> MRGSFVEMVDNLRGKSGQGYYVEMTVGSPPQTLNILVDTGSSNFAVGAAPHPFLHRYYQRQLSSTYRDLRKGVYVPYTQGKWEGELGTDLVSIPHGPNVTVRANIAAITESDKFFINGSNWEGI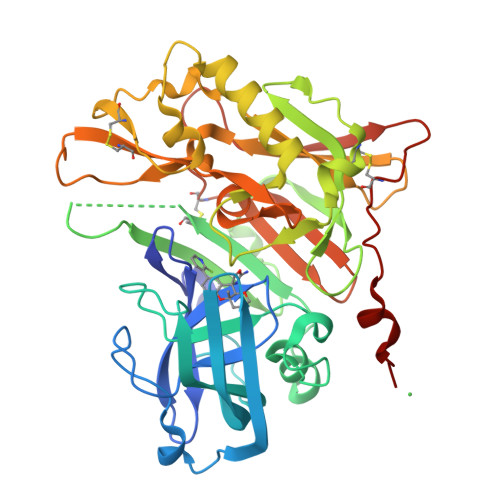LGLAYAEIARPDDSLEPFFDSLVKQTHVPNLFSLQLCGAGFPLNQSEVLASVGGSMIIGGIDHSLYTGSLWYTPIRREWYYEVIIVRVEINGQDLKMDCKEYNYDKSIVDSGTTNLRLPKKVFEAAVKSIKAASSTEKFPDGFWLGEQLVCWQAGTTPWNIFPVISLYLMGEVTNQSFRITILPQQYLRPVEDVATSQDDCYKFAISQSSTGTVMGAVIMEGFYVVFDRARKRIGFAVSACHVHDEFRTAAVEGPFVTLDMEDCGYNIPQTDESRSHHHHHH> MDQNFARNEKEAKDSAITFIQKSAAIKAGARSAEDIKLDKVNLGGELSGSNMYVYNISTGGFVIVSGDKRSPEILGYSTSGSFDANGKENIASFMESYVEQIKENKKLDTTYAGTAEIKQPVVKSLLNSKGIHYNQGNPYNL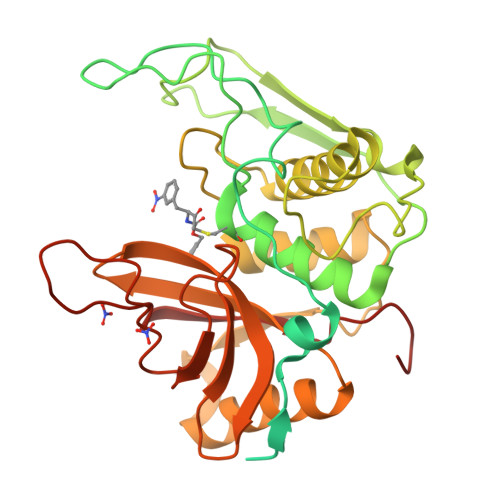LTPVIEKVKPGEQSFVGQHAATGCVATATAQIMKYHNYPNKGLKDYTYTLSSNNPYFNHPKNLFAAISTRQYNWNNILPTYSGRESNVQKMAISELMADVGISVDMDYGPSSGSAGSSRVQRALKENFGYNQSVHQINRSDFSKQDWEAQIDKELSQNQPVYYQGVGKVGGHAFVIDGADGRNFYHVNWGWGGVSDGFFRLDALNPSALGTGGGAGGFNGYQSAVVGIKPLEHHHHHH(2~{Z},6~{E})-3,7,11-trimethyldodeca-2,6-diene | C15 H28 | 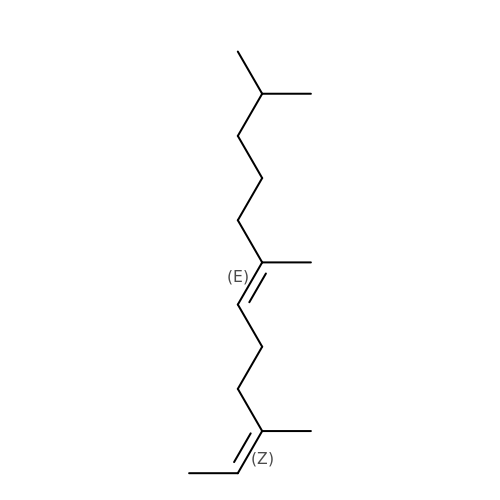JWYIGIOWHFKZIP-IBAFYIADSA-N> GSHADLLRKNAEVTKQVSMARQAQVDLEREKKELEDSLERISDQGQRKTQEQLEVLESLKQELATSQRELQVL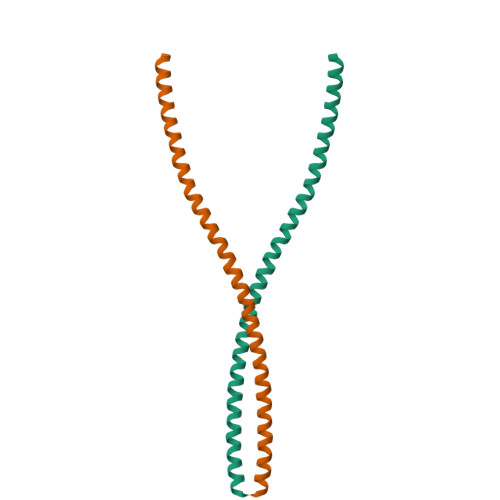QGSLETSAQSEANWAAEFAELEKERDSLVSGAAH> KVQTDPPSVPICDLYPNGVFPKGQECEYPPTQDGRTAAWRTTSEEKKALDQASEEIWNDFREAAEAHRQVRKYVMSWIKPGMTMIE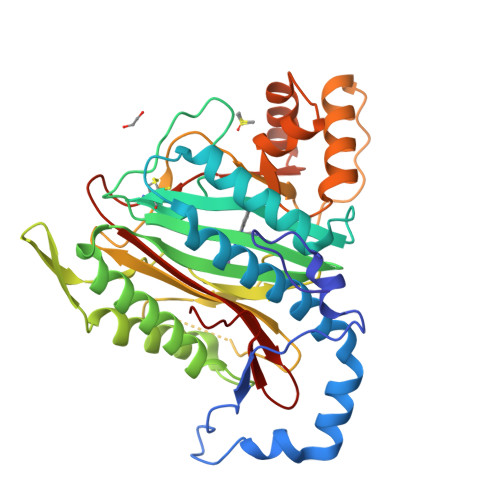ICEKLEDCSRKLIKENGLNAGLAFPTGCSLNNCAAHYTPNAGDTTVLQYDDICKIDFGTHISGRIIDCAFTVTFNPKYDTLLKAVKDATNTGIKCAGIDVRLCDVGEAIQEVMESYEVEIDGKTYQVKPIRNLNGHSIGQYRIHAGKTVPIVKGGEATRMEEGEVYAIETFGSTGKGVVHDDMECSHYMKNFDVGHVPIRLPRTKHLLNVINENFGTLAFCRRWLDRLGESKYLMALKNLCDLGIVDPYPPLCDIKGSYTAQFEHTILLRPTCKEVVSRGDDY>MPKIYTKTGDKGFSSTFTGERRPKDDQVFEAVGTTDELSSAIGFALELVTEKGHTFAEELQKIQCTLQDVGSALATPCSSAREAHLKYTTFKAGPILELEQWIDKYTSQLPPLTAFILPSGGKISSALHFCRAVCRRAER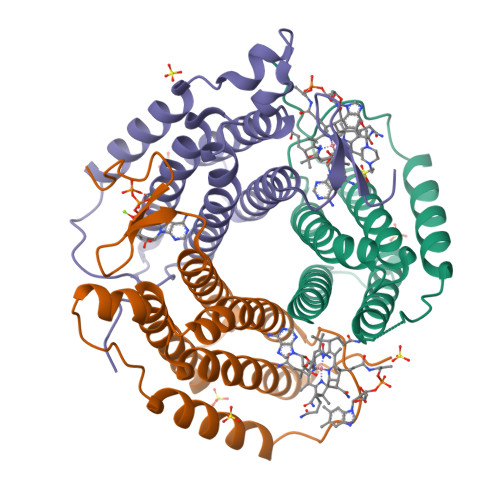RVVPLVQMGETDANVAKFLNRLSDYLFTLARYAAMKEGNQEKIYMKNDPSAESEGL[3x]>MELIRIAMKKDLENDNSLMNKWATVAGLKNPNPLYDFLNHDGKTFNEFSSIVNIVKSQYPDREYELMKDYCLNLDVKTKAARSALEYADANMFFEIEDVLIDSMISCSNMKSKEYGKVYKIHRELSNSVITEFEAVKRLGKLNIKTPEMNSFSRLLLLYHYLSTGNFSPMAQLIKQIDLSEISENMYIRNTYQTRVHVLMSNIKLNENSLEECREYSKKALESTNILRFQVFSYLTIGNSLLFSNYELAQENFLKGLSISVQNENYNMIFQQALCFLNNVWRKENKWINFESDSIMDLQEQAHCFINFNENSKAKEVLDKLDLLVHNDNELAMHYYLKGRLEQNKACFYSSIEYFKKSNDKFLIRLPLLELQKMGENQKLLELLLL[8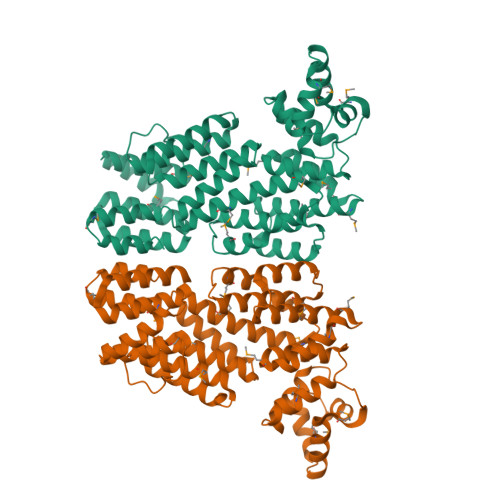x]>MDNIIMTAYISIFVQIITAIISVYGLFIPLNFKDIILREILILELIVQIIEFIFYIWLIITLQSINEDITYVRYFDWVLTTPVMLLTTVYFFEYMNSDDGIRKKEINDRDYVYLFYICLSNFFMLLIGYLGETKQINKMLTLFGGSFFLFLTFYLLYVKYTKENWMNYLVFGAMFLLWALYGFAFMFPFSIKNQ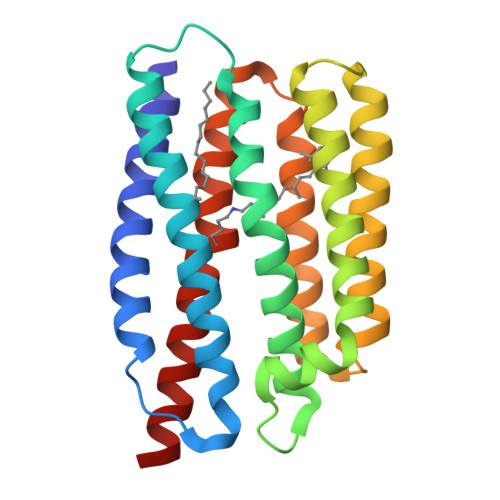MYNILDIFSKNFVSIFFFIVILNQSYKLL[2x]> MVSARKIKDNAADWHNLILKWETLNDAGFT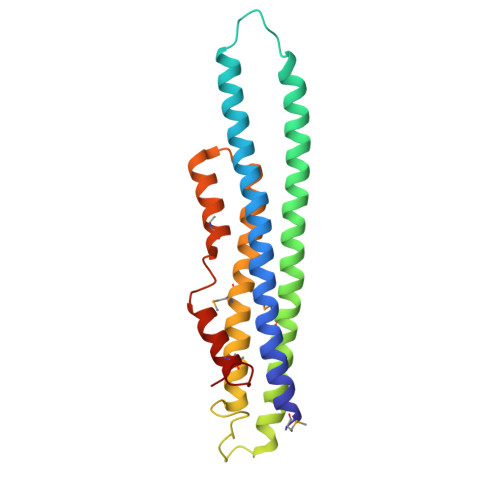TANNIANLKISLLNKDKIELDSSSPASKENEEKVCLEYNEELEKLCEELQATLDGLTKIQVKMEKLSSTTKGICELENYHYGEESKRPPLFHTWPTTHFYEVSHKLLEMYRKELLLKRTVAKELAHTGDPDLTLSYLSMWLHQPYVESDSRLHLESMLLETGHRAL> MAMHLNENLDDNGEMHDINVTPFIDVMLVLLIIFMVAAPLATVDVKVNLPASTSTPQPRPEKPVYLSVKADNSMFIGNDPVTDETMITALNALTEGKKDTTIFFRADKTVDYETLMKVMDTLHQAGYLKIGLVGEETAKAKE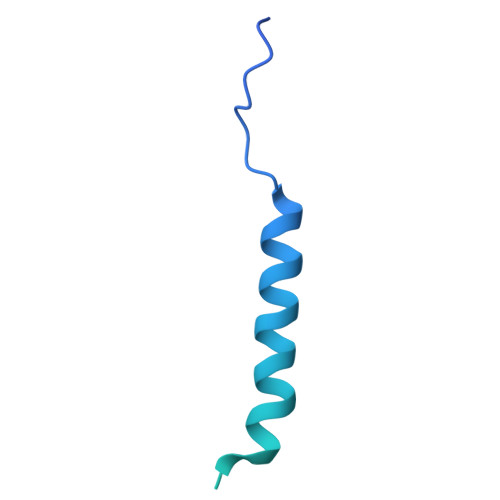NLYFQGNAGSGHHHHHHHHHH>[2x]GSHMLIYQAIKLIAQAIKVIAEAIKAIAEGDKERAKEAAEKARELYEKALELYKEAKKEGDLIAAAIALIAAAIAVIALAIAAIAAG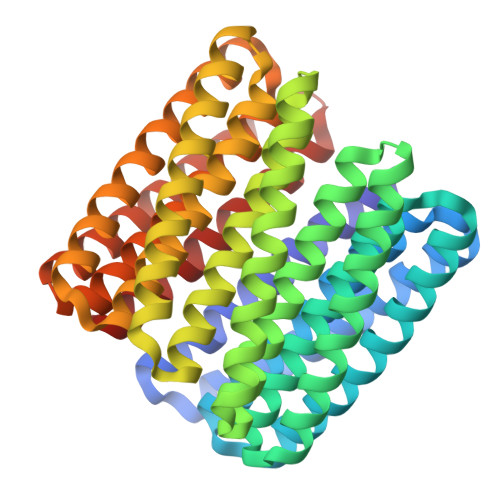DKELAKEAAELAKEIYKLAEKLYKEAKKKGDLIAAAIALIAAAIAVIALAIAAIAAGDKELAKEAAKLAKEVYKEAEELYREARKKGDLIAAAIALIAAAIAVIALAIAAIAAGDKELAKKAAELAEKVYKEALKVYKEARKKGDLIAAAIALIAAAIAVIALAIAAIAAGDKELAKKAAELAKKVLELAREIAKEARKKGDLIAAAIALIAAAIAVIALAIAAIAAGDKEEAKEAYELAKEVYKEALEIAKEARKKGDYIAAAIAAIAAAIAVIAAAIAAIAAGDKEEAKEAYKLAKEAKEKAKEIAKEAKKAGDKIAAAIAEIAQAIAEIAQAIAEIALK> EGLPPR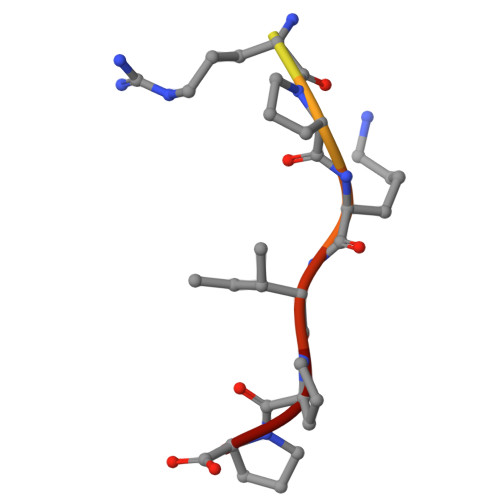PKIPP>GSMPTLLLTGFEPFHTHPDNPSAQAAQELHGLELPGGWGVHSALLPVEPHAAGAALTRLLSEQDPGAVLLTGLAAGRPQVTLERVGVGVMDFQIPDNAGQTYRDQPIEPDAPAAYLATLPLRAILAAWREAEIPGDISNSAGLYVCNFVLYHALHWLREHGRGAVPCGFLHVPANAAVALAVPADRPPLPYLPQSEITRAV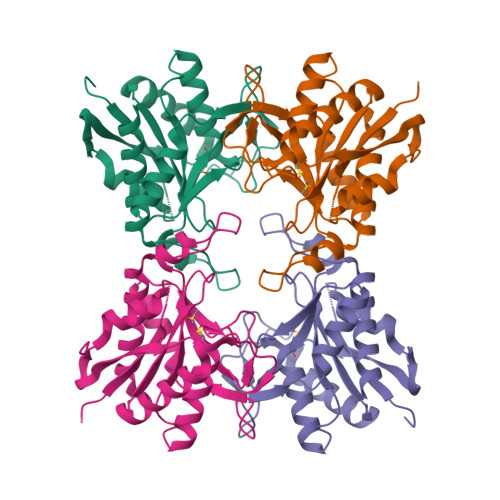RVAAEAITAQSSVLQMGKM[2x]>[12x]GSVESHPVLEKLKAAHSYNPKEFEWNLKSGRVFIIKSYSEDD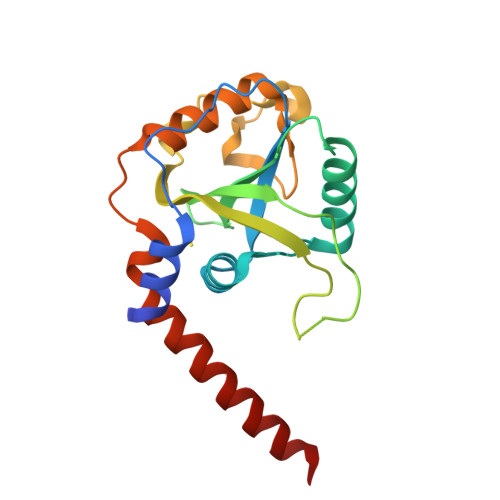IHRSIKYSIWCSTEHGNKRLDSAFRCMSSKGPVYLLFSVNGSGHFCGVAEMKSPVDYGTSAGVWSQDKWKGKFDVQWIFVKDVPNNQLRHIRLENNDNKPVTNSRDTQEVPLEKAKQVLKIISSYKHTTSIFDDFAHYEKRQAVVEVVRKERQSRNKQ> AHMAHAGRSGYDNREIVMKYIHY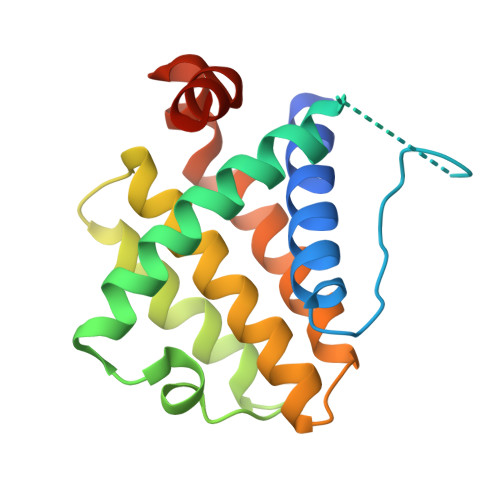KLSQRGYEWDAGDDAEENRTEAPEGTESEVVHLALRQAGDDFSRRYRRDFAEMSSQLHLTPFTARGCFATVVEELFRDGVNWGRIVAFFEFGGVMCVESVNREMSPLVDNIALWMTEYLNRHLHTWIQDNGGWDAFVELYGPSMR>[2x]GAAPDAVMVFARQGDKGSVSVGDKHFRTQAFKVRLVNAAKSEISLKNSCLVAQ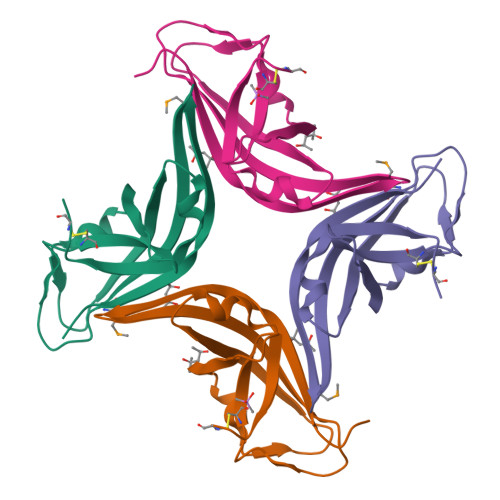SAAGQSFRLDTVDEELTADTLKPGASVEGDAIFASEDDAVYGASLVRLSDRCK The Rpd3 small (Rpd3S) complex recognizes histone H3 trimethylation on lysine 36 (H3K36me3) and deacetylates histones H3 and H4 at multiple sites across transcribed regions. The Rpd3S histone deacetylase (HDAC) complex recognizes H3K36me3 at coding regions and suppresses transcription from cryptic promoters via its deacetylase activity in yeast. Here we solved the cryo-electron microscopy structures of Saccharomyces cerevisiae Rpd3S in its free and H3K36me3 nucleosome-bound states. We demonstrated a unique architecture of Rpd3S, in which two copies of Eaf3–Rco1 heterodimers are asymmetrically assembled with Rpd3 and Sin3 to form a catalytic core complex.

Two engagement modes (‘close’ and ‘loose’) of the Rpd3S–nucleosome complexes were acquired in global density maps of 4.0 and 4.0 Å, respectively. Focused refinement led to significantly improved local maps, with 2.8 Å for the CHD–H3K36me3 nucleosome, 3.3 Å for the Rpd3S complex of the close state, and 3.4 Å for the Rpd3S complex of the loose state. The overall structure of the Rpd3S catalytic core is largely unchanged, except for poorer density of the left arm, probably owing to a lack of nucleosomal contact. Structural alignment revealed rotational displacement of the Rpd3S catalytic core from the close to the loose states, in which the MID domain of Rco1-A within the right arm leaves the linker DNA next to SHL +7 in the loose state. The nucleosomal DNA at SHL +2.5 is recognized by the HID-C region of Sin3 with multiple electrostatic or hydrogen bonding pairs involving residues Q937, K941, H1221, Q1222 and K1244 of Sin3 and backbone phosphates across the DNA minor groove. Upon engagement mode switch from the close to loose states, the H3K36me3 readout and SHL +2.5 DNA contacts act as anchoring sites to allow rotational displacement of Rpd3S, and the linker DNA contacts are temporally disrupted during the process, reflecting enzyme–substrate engagement dynamics. The existence of two engagement modes suggests dynamic association between the Rpd3S enzyme and its nucleosomal substrate, which may be beneficial for enzymatic turnover towards different acetylation sites occurred to histones H3 and H4 tails.

> MSQVWHNSNSQSNDVATSNDATGSNERNEKEPSLQGNKPGFVQQQQRITLPSLSALSTKEEDRRDSNGQQALTSHAAHILGYPPPHSNAMPSIATDSALKQPHEYHPRPKSSSSSPSINASLMNAGPAPLPTVGAASFSLSRFDNPLPIKAPVHTEEPKSYNGLQEEEKATQRPQDCKEVPAGVQPADAPDPSSNHADANDDNNNNENSHDEDADYRPLNVKDALSYLEQVKFQFSSRPDIYNLFLDIMKDFKSQAIDTPGVIERVSTLFRGYPILIQGFNTFLPQGYRIECSSNPDDPIRVTTPMGTTTVNNNISPSGRGTTDAQELGSFPESDGNGVQQPSNVPMVPSSVYQSEQNQDQQQSLPLLATSSGLPSIQQPEMPAHRQIPQSQSLVPQEDAKKNVDVEFSQAISYVNKIKTRFADQPDIYKHFLEILQTYQREQKPINEVYAQVTHLFQNAPDLLEDFKKFLPDSSASANQQVQHAQQHAQQQHEAQMHAQAQAQAQAQAQVEQQKQQQQFLYPASGYYGHPSNRGIPQQNLPPIGSFSPPTNGSTVHEAYQDQQHMQPPHFMPLPSIVQHGPNMVHQGIANENPPLSDLRTSLTEQYAPSSIQHQQQHPQSISPIANTQYGDIPVRPEIDLDPSIVPVVPEPTEPIENNISLNEEVTFFEKAKRYIGNKHLYTEFLKILNLYSQDILDLDDLVEKVDFYLGSNKELFTWFKNFVGYQEKTKCIENIVHEKHRLDLDLCEAFGPSYKRLPKSDTFMPCSGRDDMCWEVLNDEWVGHPVWASEDSGFIAHRKNQYEETLFKIEEERHEYDFYIESNLRTIQCLETIVNKIENMTENEKANFKLPPGLGHTSMTIYKKVIRKVYDKERGFEIIDALHEHPAVTAPVVLKRLKQKDEEWRRAQREWNKVWRELEQKVFFKSLDHLGLTFKQADKKLLTTKQLISEISSIKVDQTNKKIHWLTPKPKSQLDFDFPDKNIFYDILCLADTFITHTTAYSNPDKERLKDLLKYFISLFFSISFEKIEESLYSHKQNVSESSGSDDGSSIASRKRPYQQEMSLLDILHRSRYQKLKRSNDEDGKVPQLSEPPEEEPNTIEEEELIDEEAKNPWLTGNLVEEANSQGIIQNRSIFNLFANTNIYIFFRHWTTIYERLLEIKQMNERVTKEINTRSTVTFAKDLDLLSSQLSEMGLDFVGEDAYKQVLRLSRRLINGDLEHQWFEESLRQAYNNKAFKLYTIDKVTQSLVKHAHTLMTDAKTAEIMALFVKDRNASTTSAKDQIIYRLQVRSHMSNTENMFRIEFDKRTLHVSIQYIALDDLTLKEPKADEDKWKYYVTSYALPHPTEGIPHEKLKIPFLERLIEFGQDIDGTEVDEEFSPEGISVSTLKIKIQPITYQLHIENGSYDVFTRKATNKYPTIANDNTQKGMVSQKKELISKFLDCAVGLRNNLDEAQKLSMQKKWENLKDSIAKTSAGNQGIESETEKGKITKQEQSDNLDSSTASVLPASITTVPQDDNIETTGNTESSDKGAKIQ;> MVYEATPFDPITVKPSDKRRVAYFYDADVGNYAYGAGHPMKPHRIRMAHSLIMNYGLYKKMEIYRAKPATKQEMCQFHTDEYIDFLSRVTPDNLEMFKRESVKFNVGDDCPVFDGLYEYCSISGGGSMEGAARLNRGKCDVAVNYAGGLHHAKKSEASGFCYLNDIVLGIIELLRYHPRVLYIDIDVHHGDGVEEAFYTTDRVMTCSFHKYGEFFPGTGELRDIGVGAGKNYAVNVPLRDGIDDATYRSVFEPVIKKIMEWYQPSAVVLQCGGDSLSGDRLGCFNLSMEGHANCVNYVKSFGIPMMVVGGGGYTMRNVARTWCFETGLLNNVVLDKDLPYNEYYEYYGPDYKLSVRPSNMFNVNTPEYLDKVMTNIFANLENTKYAPSVQLNHTPRDAEDLGDVEEDSAEAKDTKGGSQYARDLHVEHDNEFY;> MVDLEQEFALGGRCLAFHGPLMYEAKILKIWDPSSKMYTSIPNDKPGGSSQATKEIKPQKLGEDESIPEEIINGKCFFIHYQGWKSSWDEWVGYDRIRAYNEENIAMKKRLANEAKEAKKSLLEQQKKKKLSTSLGGPSNGGKRKGDSRSNASISKSTSQSFLTSSVSGRKSGRSSANSLHPGSSLRSSSDQNGNDDRRRSSSLSPNMLHHIAGYPTPKISLQIPIKLKSVLVDDWEYVTKDKKICRLPADVTVEMVLNKYEHEVSQELESPGSQSQLSEYCAGLKLYFDKCLGNMLLYRLERLQYDELLKKSSKDQKPLVPIRIYGAIHLLRLISVLPELISSTTMDLQSCQLLIKQTEDFLVWLLMHVDEYFNDKDPNRSDDALYVNTSSQYEGVALGM;>[2x]MDTSKKDTTRSPSHSNSSSPSSSSLSSSSSKEKKRPKRLSSQNVNYDLKRRKIITSEGIERSFKNEHSNLAVEDNIPEEEPKELLEKDSKGNIIKLNEPSTISEDSKVSVTGLPLNKGPSEKIKRESLWNYRKNLGGQSNNSEMTLVPSKRFTQVPKNFQDLNRNDLKTFLTENMTEESNIRSTIGWNGDIINRTRDREPESDRDNKKLSNIRTKIILSTNATYDSKSKLFGQNSIKSTSNASEKIFRDKNNSTIDFENEDFCSACNQSGSFLCCDTCPKSFHFLCLDPPIDPNNLPKGDWHCNECKFKIFINNSMATLKKIESNFIKQNNNVKIFAKLLFNIDSHNPKQFQLPNYIKETFPAVKTGSRGQYSDENDKIPLTDRQLFNTSYGQSITKLDSYNPDTHIDSNSGKFLICYKCNQTRLGSWSHPENSRLIMTCDYCQTPWHLDCVPRASFKNLGSKWKCPLHSPTKVYKKIHHCQEDNSVNYKVWKKQRLINKKNQLYYEPLQKIGYQNNGNIQIIPTTSHTDYDFNQDFKITQIDENSIKYDFFDKIYKSKMVQKRKLFQFQESLIDKLVSNGSQNGNSEDNMVKDIASLIYFQVSNNDKSSNNKSASKSNNLRKLWDLKELTNVVVPNELDSIQFNDFSSDEIKHLLYLKKIIESKPKEELLKFLNIENPENQSE> TTLLNPYFGEFGGMYVPQILMPALNQLEEAFVSAQKDPEFQAQFADLLKNYAGRPTALTKCQNITAGTRTTLYLKREDLLHGGAHKTNQVLGQALLAKRMGKSEIIAETGAGQHGVASALASALLGLKCRIYMGAKDVERQSPNVFRMRLMGAEVIPVHSGSATLKDACNEALRDWSGS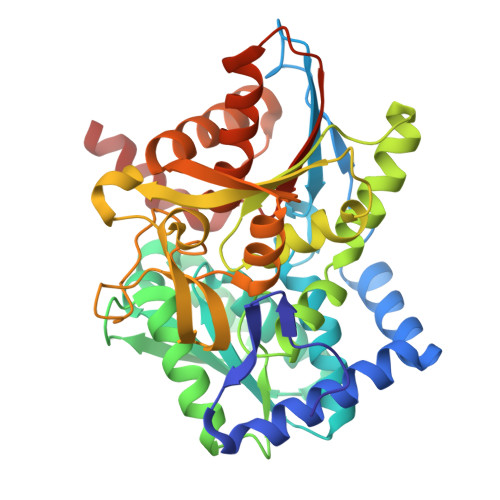YETAHYMLGTAAGPHPYPTIVREFQRMIGEETKAQILDKEGRLPDAVIACVGGGSNAIGMFADFINDTSVGLIGVEPGGHGIETGEHGAPLKHGRVGIYFGMKAPMMQTADGQIEESYSISAGLDFPSVGPQHAYLNSIGRADYVSITDDEALEAFKTLCRHEGIIPALESSHALAHALKMMREQPEKEQLLVVNLSGRGDKDIFTVHDILKARGEI> GAMESLPVIAAPSMWTRPQIKDFKEKIQQDADSVITVGRGEVVTVRVPTHEEGSYLFWEFATDNYDIGFGVYFEWTDSPNTAVSVHVSESSDDDEEEEENIGCEEKAKKNANKPLLDEIVPVYRRDCHEEVYAGSHQYPGRGVYLLKFDNSYSL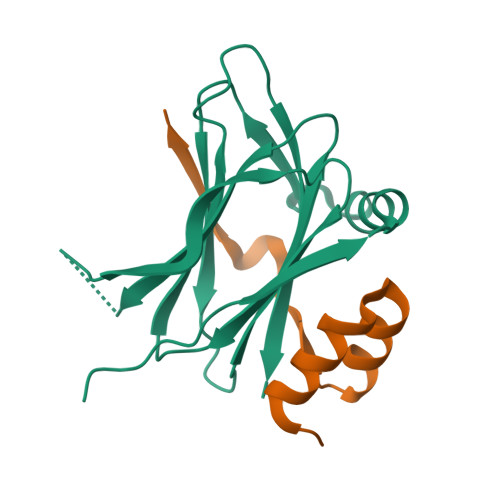WRSKSVYYRVYYTR;> GSGSGTPAPDAINDLLRSVDSQEVRDYCQKKGWIVIHPSNELVVEKHISR> DVSTSYLRHNEINEYLQTLSQKYPSLVSVEEAGTSYEGRSIKTITINKKPGNAVVFLDAGIHAREWIAPATALYAIEQLVEHSSENQEVLSNLTWVIMPVVNPDGYEFSHETDRFWRKTRKPTGKSCKGTDGNRNFDYHWGEVGASTQACADTFRGETAFSEPETRAVRDAVMKLKGSCKFYLSLHSYGNYILYPWGWTSKLPETWEAIDEVAQAGAEAIKQSTGSRYTVGSSTNVLYAAAGGSDDWAFAVAEVPISITMELPGGGNGGFNPPPSSIEKIVNESWVGI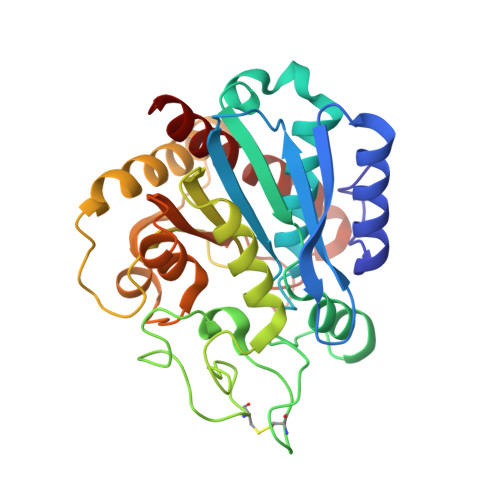KAMALKVAQMF Here we present a strategy for fusing small RNAs to a group II intron that yields high resolution structures of the appended RNA. Group II introns are self-splicing catalytic RNAs that have six distinct domains and typically range in size from 400 to 850 nucleotides. Our versatile scaffolding strategy enables efficient RNA structure determination for a broad range of small to moderate-sized RNAs, which were previously intractable for high-resolution cryo-EM studies.

The TPP riboswitch binds to thiamine pyrophosphate and modulates gene expression, with a wide phylogenetic distribution in both prokaryotes and eukaryotes. We then performed local refinement on the riboswitch component, which yielded a reconstruction with a global resolution of 3.1 Å, and 2.5 Å for the ligand-binding pocket. The viewing distribution plot shows that embedding the riboswitch did not create a preferred orientation for the overall fusion construct. This resolution yielded clear density for the functional groups in this small molecule and enabled modeling of the TPP ligand with high confidence. Density for three magnesium ions, coordinated to the pyrophosphate moiety, are clearly visible. Only two metal ions were visualized binding to the pyrophosphate in previous crystal structures. These magnesium ions are essential for binding of TPP to this riboswitch. In contrast, upon ligand binding, the RNA adopts a compact tertiary structure in which these two stems are parallel to each other and the P3 and L5 motifs form a long-range tertiary interaction, stabilizing the binding pocket for TPP. When TPP is bound (right), the P3-L5 interaction is engaged, and the riboswitch compacts leading to ordered P1, J2-4, and P4 regions (circled red) forming a compact three-way junction. For the TPP riboswitch, the resolution observed here is the highest ever achieved by cryo-EM for an RNA less than 100 nucleotides.

> UUAUGUGUGCCCGGCAUGGGUGCAGUCUAUAGGGUGAGAGUCCCGAACUGUGAAGGCAGAAGUAACAGUUAGCCUAACGCAAGGGUGUCCGUGGCGACAUGGAAUCUGAAGGAAGCGGACGGCAAACCUUCGGUCUGAGGAACACGAACUUCAUAUGAGGCUAGGUAUCAAUGGAUGAGUUUGCAUAACAAAACAAAGUCCUUUCUGCCAAAGUUGGUACAGAGUAAAUGAAGCAGAUUGAUGAAGGGAAAGACUGCAUUCUUACCCGGGGAGGUCUGGAAACAGAAGUCAGCAGAAGUCAUAGUACCCUCAGUACUCGGGGUGCCCUUCUGCGUGAAGGCUGAGAAAUACCCGUAUCACCUGAUCUGGAUAAUGCCAGCGUAGGGAAGUGCUGAGGGGAAGGACGGAACAAGUAUGGCGUUCGCGCCUAAGCUUGAACCACCGUAUACCGAACGGUACGUACGGUGGUGUGAGAGGAGUUCGCUCUACUCUAUUAG> ELGDSLEEFLAKATTDKNLARLLVCMGEALRTIAFKVRTASCGATACTNTFGDEQLAVDMLADKLLFE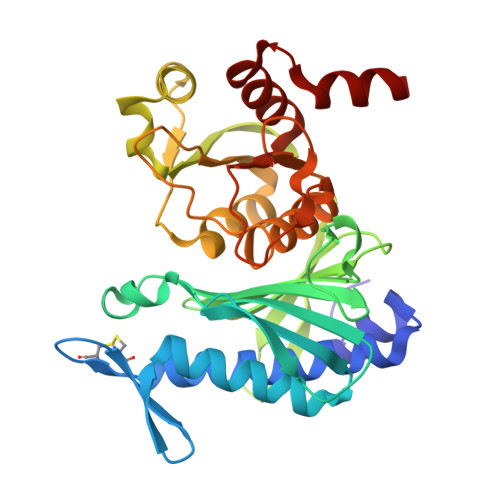ALRHSHVCKYACSEEEPILQDMEGEGFSVAFDPLDGSSIVDTNFTVGTIFGVWPGDKLTGITGRDQAASAMGIYGPRTTYVVAINGFPGTHEFLLMDDGKWQHVKETTEIKEGKLFSPGNLRATFDNADYEKLINYYVSEKYTLRYTGGMVPDVNQIIVKERGIFTNVTSPTTKAKLRLLFEVAPLGLLIENAGGYSSDGKQSVLDKVVVNTDDRTQVAYGSRDEIIRFEETLYGDSRLKAELAATVV Here, we report six structures with near-atomic resolution captured by cryo-EM, representing human Eag2 (hEag2) in closed, pre-open, open, and pore dilation but non-conducting states. We expressed full-length hEag2 fused with a green fluorescent protein (GFP) in HEK293T cells and characterized its electrophysiological properties and show that it is a voltage-activated delayed rectifier potassium channel with a half-activation membrane potential of −10.0 ± 3.5 mV. The channel has a three-layer architecture: the upper extracellular turret, transmembrane domains, and intracellular domains occupying 3D space with a size of 130 Å × 130 Å × 130 Å. The tetrameric hEag2 apparatus adopts noncanonical non-domain-swapped VSDs, with distinct pore domain configurations.

The overall Cα atoms and the side chain of the two closed states are almost identical, while the differences are density peaks of the water molecule and potassium ion in S0, indicating that the water and potassium in S0 layer are dynamic in the closed states. For hEag2, in a closed state, the four pore-lining S6 helices form a bundle-crossing in the middle of the membrane right below the ion selectivity filter with two layers of hydroxyphenyl or phenyl residue, Y460s and F464s, forming the hydrophobic constriction sites through intrachain and interchain π–π interaction to prevent hydrated/dehydrated potassium ion flow. Below the hydrophobic constriction sites are hydrophilic constriction sites through intrachain and interchain electrostatic interaction of Q472s and T468s. The hydrophilic constriction sites together with the hydrophobic ones form a long channel gate. In the closed states and pre-open state 1, a strong and unambiguous density peak is located between the hydrophobic and hydrophilic constriction sites. The density is more likely to be a dehydrated potassium ion, and we name it site 6 or S6 as the seventh potassium ion selectivity site.

>[4x]MPGGKRGLVAPQNTFLENIVRRSSESSFLLGNAQIVDWPVVYSNDGFCKLSGYHRADVMQKSSTCSFMYGELTDKKTIEKVRQTFDNYESNCFEVLLYKKNRTPVWFYMQIAPIRNEHEKVVLFLCTFKDITLFKQPIEDDSTKGWTKFARLTRALTNSRSVLQQLTPMNKTEVVHKHSRLAEVLQLGSDILPQYKQEAPKTPPHIILHYCAFKTTWDWVILILTFYTAIMVPYNVSFKTKQNNIAWLVLDSVVDVIFLVDIVLNFHTTFVGPGGEVISDPKLIRMNYLKTWFVIDLLSCLPYDIINAFENVDEGISSLFSSLKVVRLLRLGRVARKLDHYLEYGAAVLVLLVCVFGLVAHWLACIWYSIGDYEVIDEVTNTIQIDSWLYQLALSIGTPYRYNTSAGIWEGGPSKDSLYVSSLYFTMTSLTTIGFGNIAPTTDVEKMFSVAMMMVGSLLYATIFGNVTTIFQQMYANTNRYHEMLNNVRDFLKLYQVPKGLSERVMDYIVSTWSMSKGIDTEKVLSICPKDMRADICVHLNRKVFNEHPAFRLASDGCLRALAVEFQTIHCAPGDLIYHAGESVDALCFVVSGSLEVIQDDEVVAILGKGDVFGDIFWKETTLAHACANVRALTYCDLHIIKREALLKVLDFYTAFANSFSRNLTLTCNLRKRIIFRKISDVKKEEEERLRQKNEVTLSIPVDHPVRKLFQKFKQQKELRNQGSTQGDPERNQLQVESRSLQNGASITGTSVVTVSQITPIQTSLAYVKTSESLKQNNRDAMELKPNGGADQKCLKVNSPIRMKNGNGKGWLRLKNNMGAHEEKKEDWNNVTKAESMGLLSEDPKSSDSENSVTKNPLRKTDSCDSGITKSDLRLDKAGEARSPLEHSPIQADAKHPFYPIPEQALQTTLQEVKHELKEDIQLLSCRMTALEKQVAEILKILSEKSVPQASSPKSQMPLQVPPQIPCQDIFSVSRPESPESDKDEIHF>[4x]SEFELGAPAGRQAGQQATVDRLRTQVTGFLSGALGKLQALSAQNMDPELAQFRVLDVDRAIMPLLIVAENARNPGLNLVPLHMDMAEDEEVRTQPPMAGSRHIAEFVASARPG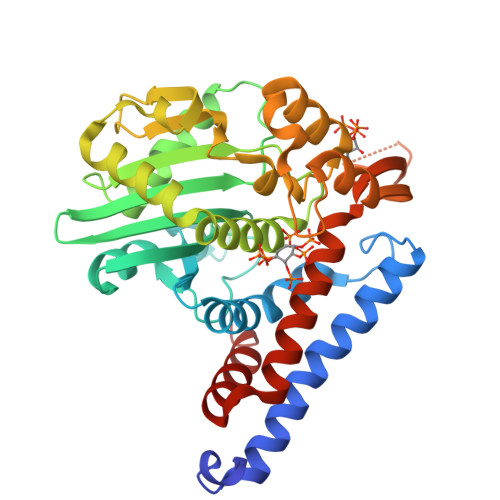RYRAVIDDGSHTRAADIRKDASGTSVIVVDPLRKEKDESAYVDYADNVNMEFGEHAKCAFIPVDIQKSFFDARILSLSLALKMHDKDDAFAAFHETLRNGGDPSHHVSRAQQTEELGATLVLDGAPLVDARMMKHGQAASSVSRYLGNHPEQSTVPVNKRNETLGERTTRHLVKRKVRNRADSEGRVTSGETKEITFSNSVEQKRIALLNRAASYVNSAPPPVVMRMAKLLQDSLLDTN1-nitrooctane | C8 H17 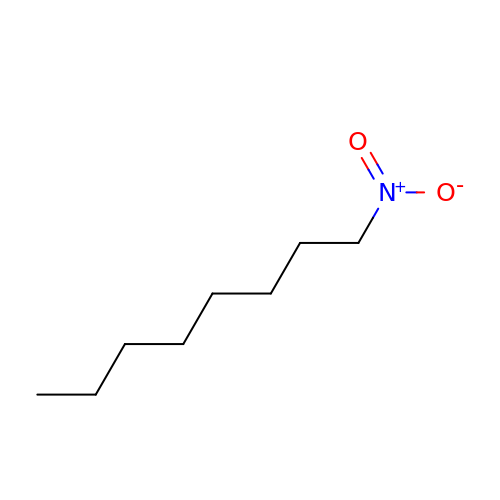N O2 | KLGHUFNKRIWCDQ-UHFFFAOYSA-N>MSLSQDGLLGEVLSEGVLTLTLGRAPAHPLSRAMIAALHDALRRAMGDDHVHVLVIHGPGRIFCAGHDLKEIGRHRADPDEGRAFVTDLFEACSALMLDLAHCPKPTIALVEGIATAAGLQLMAA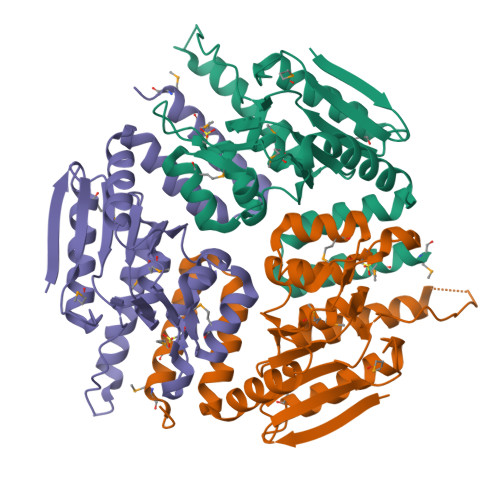CDLAYASPAARFCLPGVQNGGFCTTPAVAVSRVIGRRAVTEMALTGATYDADWALAAGLINRILPEAALATHVADLAGALAARNQAPLRRGLETLNRHLELPLEQAYALATPVMVEHFMDPGRRHLDWIDEGHHHHHH[12x]> MTTQLRYENNDDDERVEYNLFTNRSTMMANFEEWIKMATDNKINSRNSWNFALIDYFYDLDVLKDGENNINFQKASATLDGCIKIYSSRVDSVTTETGKLLSGLAQRKTNGASNGDDSNGGNGEGLGGDSDEANIEIDPLTGMPISNDPDVNNTRRRVYNRVLETTLVEFETIKMKELDQELIIDPLFKKALVDFDEGGAKSLLLNTLNIDNTARVIFDASIKDTQNVGQGKLQRKEEELIERDSLVDDENEPSQSLISTRNDSTVNDSVISAPSMEDEILSLGMDFIKFDQIAVCEISGSIEQLRNVVEDINQAKDFIENVNNRFDNFLTEEELQAAVPDNAEDDSDGFDMGMQQELCYPDENHDNTSHDEQDDDNVNSTTGSIFEKDLMAYFDENLNRNWRGREHWKVRNFKKANLVNKESDLLEETRTTIGDTTDKNTTDDKSMDTKKKHKQKKVLEIDFFKTDDSFEDKVFASKGRTKIDMPIKNRKNDTHYLLPDDFHFSTDRITRLFIKPGQKM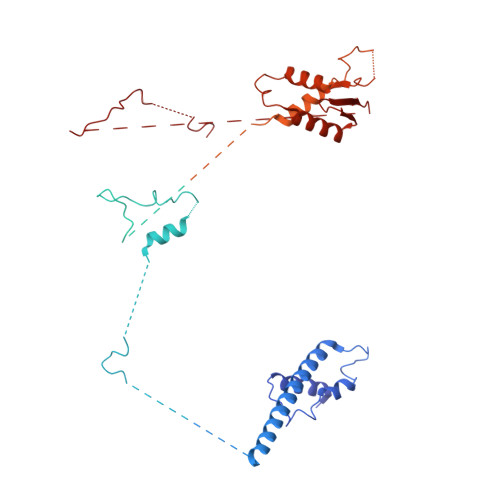SLFSHRKHTRGDVSSGLFEKSTVSANHSNNDIPTIADEHFWADNYERKEQEEKEKEQSKEVGDVVGGALDNPFEDDMDGVDFNQAFEGTDDNEEASVKLDLQDDEDHKFPIRENKVTYSRVSKKVDVRRLKKNVWRSINNLIQEHDSRKNREQSSNDSETHTEDESTKELKFSDIIQGISKMYSDDTLKDISTSFCFICLLHLANEHGLQITHTENYNDLIVNYEDLATTQAASXXXXXXXXXXXXXXXXXXX>[8x]MTMASVPASRYLTDMTLEEMSRDWSMLIPKQKVAGPLCIRMDQAIMDKNIILKANFSVIFDRLETLILLRAFTEEGAIVGEISPLPSLPGHTAEDVKNAVGVLIGGLEWNDNTV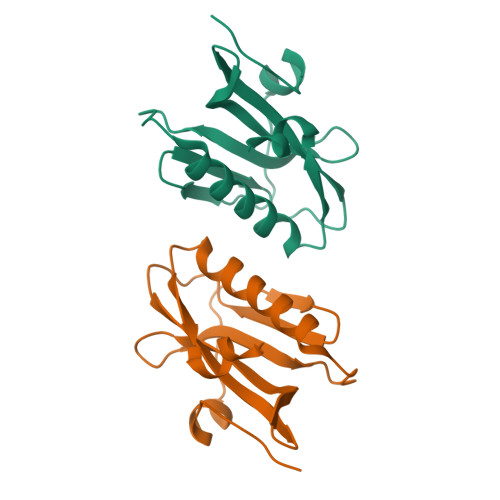RVSETLQRFAWRSSNENGRPPLTPKQKREMAGTIRSEV Here we describe a new mechanism by which foot-and-mouth disease virus (FMDV) can become resistant to ribavirin. Amino acid changes in the viral polymerase, selected by ribavirin, are able to modify the types of mutations produced in the presence of ribavirin. P44S but not P169S was detected in a 70% proportion in R-Ap35, as evidenced by analysis of both the consensus sequences and their corresponding mutant spectra. These results suggest that the three substitutions in 3D were selected sequentially during replication in the presence of increasing concentrations of R: first M296I, then P44S and finally P169S. To identify possible structural modifications of the viral polymerase associated with the important alterations of the mutational spectrum in progeny RNA, and to investigate how these modifications can affect RNA binding and polymerase activity, the different mutant 3Ds were incubated with the heteropolymeric sym/sub-U RNA of sequence 5′GCAUGGGCCC3′, crystallized, and analyzed by X-ray diffraction.

Two different crystal forms were obtained; the single mutants 3D(P44S) and 3D(P169S) incubated with sym/sub-U RNA crystallized in the tetragonal P42212 space group. The RNA molecule appeared mostly disordered in the two structures. The X-ray structures were determined to 2.2 Å and 2.6 Å resolution for 3D(P44S) and 3D(P169S), respectively, and to 2.6 Å and 2.5 Å for 3D(P44S, M296I) and 3D(SSI), respectively. P44 is conserved among known picornaviral polymerases, and it lies in a loop that connects strand β2 and helix α2 in the fingers domain. Thus, substitutions at the conserved amino acid P44 might disturb both the shape and interactions of the template channel, and the interactions with the incoming rNTP that are mediated by residues of motif F. Interestingly, the amino acid residues from M16 to K18, at the N-terminus of the enzyme, appear totally re-organized. The rearrangements in M16-K18 were also observed in the uncomplexed 3D(P44S), but with a weak electron density and higher temperature factors than the average, reflecting some degree of flexibility of this region in the absence of RNA. Thus, the structural results point at P44S as the key substitution related to reorientation of template residues that might be associated with altered RMP recognition and incorporation. The comparison of activity values in vitro suggests that amino acid P44S inflicted a cost upon 3D function. 3D(P44S) displayed undetectable incorporation of RMP opposite C in the template (<0.5% of elongated sym/sub-AC), and only a modest incorporation opposite U (5±1% of elongated sym/sub-AU).

> GLIVDTRDVEERVHVMRKTKLAPTVAHGVFNPEFGPAALSNKDSRLNEGVVLDEVIFSKHKGDTKMSAEDKALFRRCAADYASRLHSVLGTANAPLSIYEAIKGVDGLDAMEPDTAPGLPWALQGKRRGALIDFENGTVGPEVEAALKLMEKREYKFACQTFLKDEIRPMEKVRAGKTRIVDVLPVEHILYTRMMIGRFCAQMHSNNGPQIGSAVGCNPDVDWQRFGTHFAQYRNVWDVDYSAFDANHCSDAMNIMFEEVFRTEFGFHPNAEWILKTLVNTEHAYENKRITVEGGMPSGCSATSIINTILNNIYVLYALRRHYEGVELDTYTMISYGDDIVVASDYDLDFEALKPHFKSLGQTITPADKSDKGFVLGHSITDVTFLKRHFHMDYGTGFYKPVMASKTLEAILSFARRGTIQEKLISVAGLAVHSGPDEYRRLFEPFQGLFEIPSYRSLYLRWVNAVCGDAAAAEHH>MTTYSNKGPKPERGRFLHFHSVTFWVGNAKQAASFYCNKMGFEPLAYKGLETGSREVVSHVIKQGKIVFVLCSALNPWNKEMGDHLVKHGDGVKDIAFEVEDCEHIVQKARERGAKIVREPWVEEDKFGKVKFAVLQTYGDTTHTLVEKINYTGRFLPGFEAPTYKDTLLPKLPSCNLEIIDHIVGNQPDQEMESASEWYLKNLQFHRFWSVDDTQVHTEYSSLRSIVVANYEESIKMPINEPAPGRKKSQIQEYVDYNGGAGVQHIALRTEDIITTIRHLRERGMEFLAVPSSYYRLLRENLKTSKIQVKENMDVLEELKILVDYDEKGYLLQIFTKPMQDR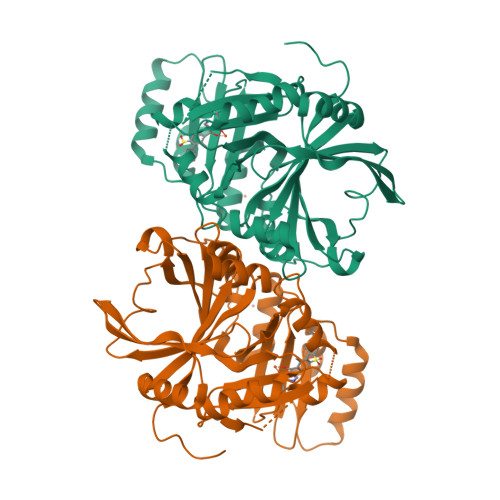PTLFLEVIQRHNHQGFGAGNFNSLFKAFEEEQALRGNLTDLETNGVRSGM[2x]>[2x]MGKVNVAKLRYMSRDDFRVLTAVEMGMKNHE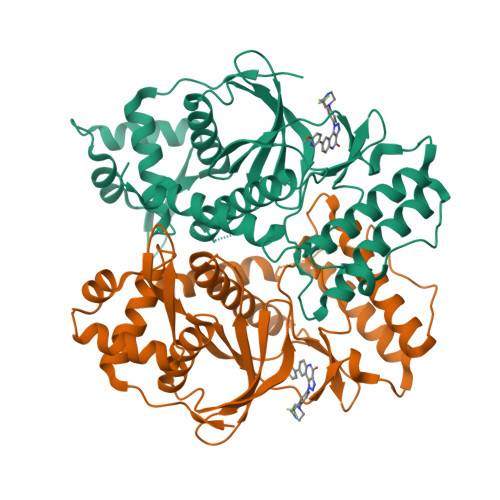IVPGSLIASIASLKHGGCNKVLRELVKHKLIAWERTKTVQGYRLTNAGYDYLALKTLSSRQVVESVGNQMGVGKESDIYIVANEEGQQFALKLHRLGRTSFRNLKNKRDYHKHRHNVSWLYLSRLSAMKEFAYMKALYERKFPVPKPIDYNRHAVVMELINGYPLCQIHHVEDPASVYDEAMELIVKLANHGLIHGDFNEFNLILDESDHITMIDFPQMVSTSHPNAEWYFDRDVKCIKDFFMKRFSYESELFPTFKDIRREDTLDVEVSASGYTKEMQADDELLHPL> STMEN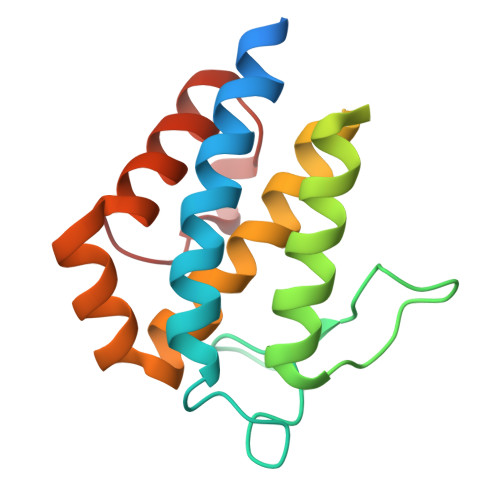IDKILEPPEGQDEGVWKYEHLRQFCLELNGLAVKLQSECHPDTCTQMTATEQWIFLCAAHKTPKECPAIDYTRHTLDGAACLLNSNKYFPSRVSIKESSVAKLGSVCRRIYRIFSHAYFHHRQIFDEYENETFLCHRFTKFVMKYNLMSKDNLIVPI>[2x]SGSKISMALQSKAVKSISDADDEILLSANEKRWLDEGNGRVLLFQLSGPMIFGVAKAIAREHNAIQECAAIVFDLSDVPHLGVDASLALENAI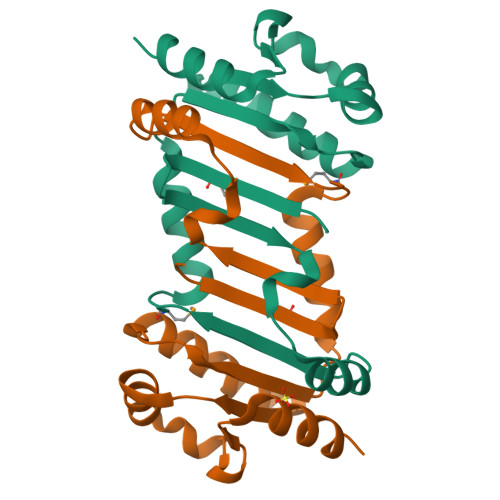EEAAEKGRAVYIVGATGQTKRRLEKLQVFRFVPESNCYDDRSEALKDAVLALGPHESEDSPSSSSVQTTY~{N}-butyl-4-chloranyl-2-(2-phenylethylsulfanyl)-5-sulfamoyl-benzamide 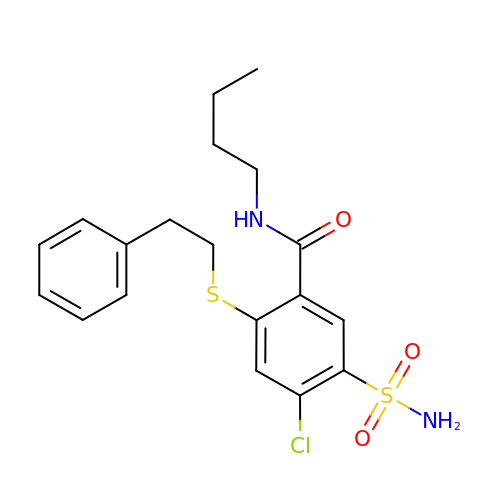| C19 H23 Cl N2 O3 S2 | GKEVLRUIWRFAPB-UHFFFAOYSA-N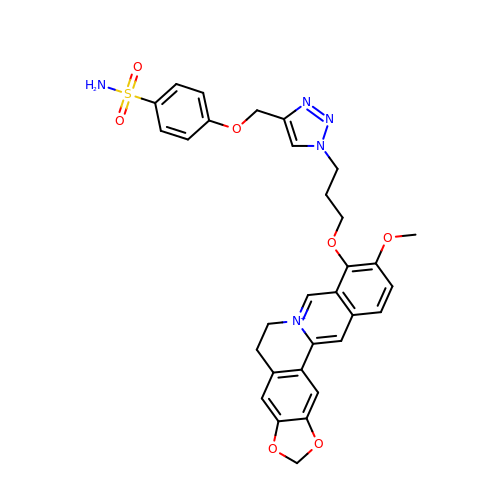4-[[1-[3-[(17-methoxy-5,7-dioxa-13-azoniapentacyclo[11.8.0.0^{2,10}.0^{4,8}.0^{15,20}]henicosa-1(21),2(10),3,8,13,15,17,19-octaen-16-yl)oxy]propyl]triazol-4-yl]methoxy]benzenesulfonamide | C31 H30 N5 O7 S | ZPZQYKHNQSCVCG-UHFFFAOYSA-N>[4x]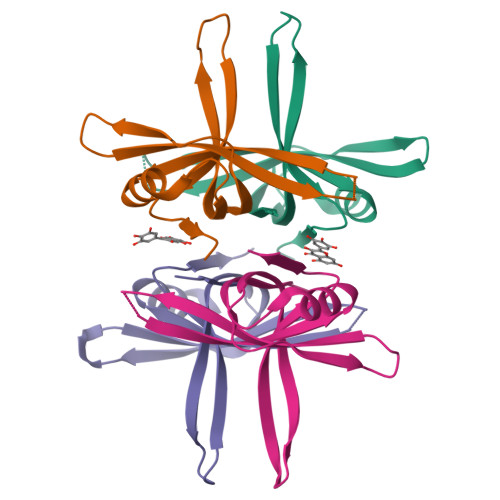MARGVNKVILVGNVGGDPETRYMPNGNAVTNITLATSESWKDKQTGQQQERTEWHRVVFFGRLAEIAGEYLRKGSQVYVEGSLRTRKWQGQDGQDRYTTEIVVDINGNMQLLGGRHHHHHH> LEEKKVCQGTSNKLTQLGTFEDHFLSLQRMFNNCEVVLGNLEITYVQRNYDLSFLKTIQEVAGYVLIALNTVERIPLENLQIIRGNMYYENSYALAVLSNYDANKTGLKELPMRNLQEILHGAVRFSNNPALCNVESIQWRDIVSSDFLSNMSMDFQNHLGSCQKCDPSCPNGSCWGAGEENCQKLTKIICAQQCSGRCRGKSPSDCCHNQCAAGCTGPRESDCLVCRKFRDEATCKDTCPPLMLYNPTTYQMDVNPEGKYSFGVTCVKKCPRNYVVTDHGSCVRACGADSYEMEEDGVRKCKKCEGPCRKVCNGIGIGEFKDSLSINATNIKHFKNCTSISGDLHILPVAFRGDSFTHTPPLDPQELDILKTVKEITGFLLIQAWPENRTDLH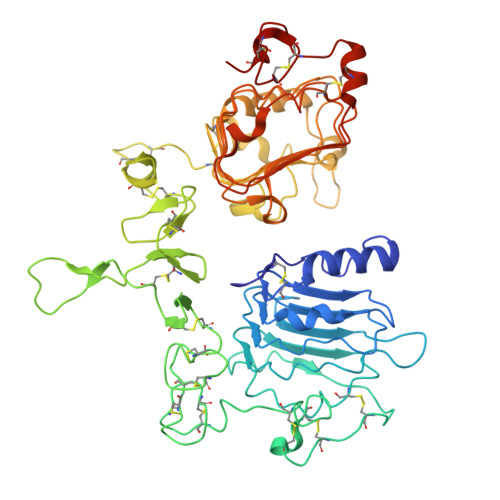AFENLEIIRGRTKQHGQFSLAVVSLNITSLGLRSLKEISDGDVIISGNKNLCYANTINWKKLFGTSGQKTKIISNRGENSCKATGQVCHALCSPEGCWGPEPRDCVSHHHHHH> MRAGIRKALIDNIKELKGCYEPNVPNKDTKKPYMVVVQGQDNDHGETIGFERSIEVWIYEGRTTFKKLDKLTKQVVEVLDMNTIVDESENEAFTCIYKGTSENDIVVEEWDAIARGIRFSVIALEDKEDTT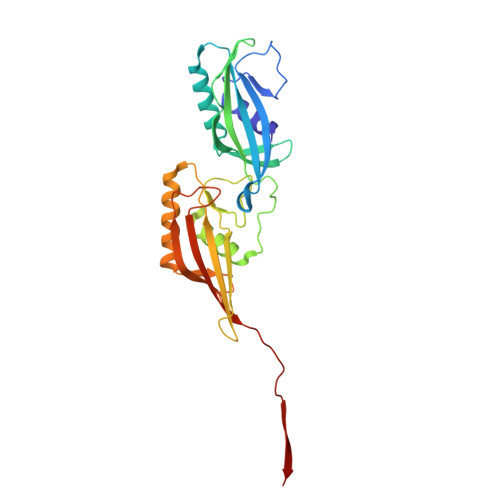NDRWVEALSRHTKDLLEIESYKDNWKKNFIAPCALWRTTHIENKRINYHLIEITKTMKCHVVSKNKDEIVKLLETLETSLIIDKRVRLREDKNMYLTLVSVVEDRESDMFTTGQLTAVFKMIGKIKREGPTMDKIYGNGNLK> MAKDELPIVNPEETGNLTDWDNEPTVSDLKSDYDSAYSSHSAQMSQITTWLNNLNVEGSAKPKKVPGRSSVQPMLIRKQAEWRYSALTEPFLSTDELFAVSPVTWEDREAAIQNQLVLNYQFNIKIDKVRFIDDYVRNAVNEGTVIVRVGWCNYTQMVKETVPVYAYYPAANEDQVAALQEALQLKLENPNAYNSLPDDIIASVDYSFENRGAFVAVQTGTEEVEYEKVIKNQPTVEVVNSQNVVIDPTCNGDISQAQFVIYSFETSKSDLEKDGRYKNLDKISASMSNPLNTPDHQ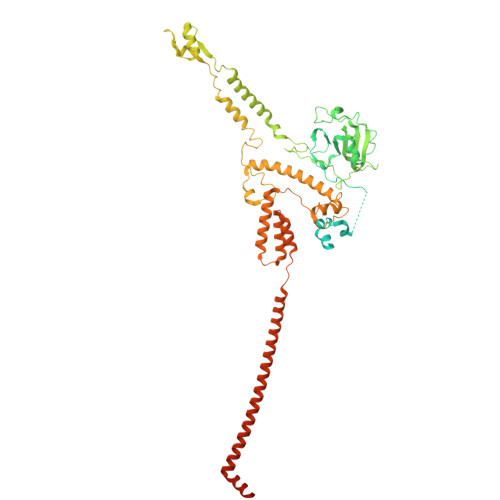VEDQSGFNFKDEPRKKFVAYEYWGWWDINGNGKTVPIVATFVGNTMIRLEENPFPDKKIPFVVVPYLPVPRSIYGEPDGALLEDNQKIIGATTRAMIDILARSANGQTGIRKDMLDVTNRRKFDKGEDYEFNANVDPRQGIYMHVSPEIPQSAPMMIQYQNNEAESLTGVKSFSQGIASQALGDVAAGIRGALDAASKRELGILRRLAQGVVEIGRKIISMNSEFLSEEEVVRVTNEQFVTVRRDELAGEFDLKLSISTAEADNQKAQELAFMLQTMGNSLPFEMSQMVLSDIARLRNMPDLAKRIESYQPQPDPLAQRKAELEIALLEAQIAETQSKAIENRASAGYKATQAQNVQSDTDLKNLDYVEQESGVKQARDVQKISAQAESQTQTKIVDYILKSGKPLSEI>[8x]MAVESRSRVTSKLVKAHRAMLNSVTQEDLKVDRLPGADYPNPSKKYSSRTEFRDKTDYIMYNPRPRDEPSSENPVSVSPLLCELAAARSRIHFNPTETTIGIVTCGGICPGLNDVIRSIT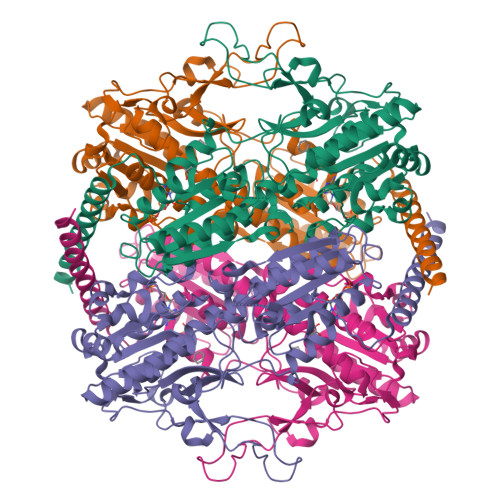LTGINVYNVKRVIGFRFGYWGLSKKGSQTAIELHRGRVTNIHHYGGTILGSSRGPQDPKEMVDTLERLGVNILFTVGGDGTQRGALVISQEAKRRGVDISVFGVPKTIDNDLSFSHRTFGFQTAVEKAVQAIRAAYAEAVSANYGVGVVKLMGRDSGFIAAQAAVASAQANICLVPENPISEQEVMSLLERRFCHSRSCVIIVAEGFGQDWGRGSGGYDASGNKKLIDIGVILTEKVKAFLKANKSRYPDSTVKYIDPSYMIRACPPSANDALFCATLATLAVHEAMAGATGCIIAMRHNNYILVPIKVATSVRRVLDLRGQLWRQVREITVDLGSDVRLARKLEIRRELEAINRNRDRLHEELAKL(5E)-5-[(N-tert-butoxycarbamimidoyl)imino]-L-norvaline | C10 H20 N4 O3 | 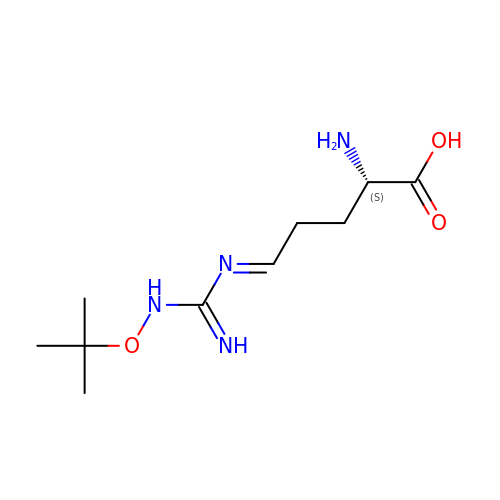TUOBZAXIKVQKKU-PQHBYJLHSA-N> MSAIKPDMKIKLRMEGNVNGHHFVIDGDGTGKPFEGKQSMDLEVKEGGPLPFAFDILTTAFXNRVFAKYPDNIQDYFKQSFPKGYSWERSLTFEDGGICNARNDITMEGDTFYNKVRFYGTNFPANGPVMQKKTLKWEPSTEKMYVRDGVLTGDVETALLLEGNAHYRCDFRTTYKAKEKGVKLPGAHFVDHCIEILSHDKDYNKVKLYEHAVAHSGLPN

The system studied was a reversibly switchable fluorescent protein (rsFP) which is a representative of a class of proteins that undergo a reversible photolysis reaction from a highly fluorescent “on” state to a weakly fluorescence “off” state. The specific rsFP used, rsKiiro, is a mutant of Skylan-NS33 specifically developed for ultrafast time-resolved crystallographic studies due to its ability to form crystals that diffract to high resolution (∼1.1 Å for single-crystal cryo-MX), high photoswitching quantum yield (∼18% Trans-to-Cis in the crystal), and high protein expression yields. Structurally, rsKiiro is similar to green fluorescent protein (GFP) with an 11-stranded β-barrel surrounding an α helix. The chromophore of rsKiiro is formed from the Ala-Tyr-Gly tripeptide at residue numbers 62–64 in the α helix.

In this study, we probed the light-induced reverse reaction, from the Trans to Cis chromophore conformation, initiated with 2 ms 405 nm pulses at a range of optical flash energy densities (0.1–6.7 mJ/mm2) after the initial Cis-to-Trans photoconversion had been driven to completion using ∼13 mW/mm2 of 473 nm CW illumination. A total of 435,200 images were obtained across 6 laser energy densities at 405 nm of 0, 0.1, 0.53, 1.78, 6.74, and 14.43 mJ/mm2. In the preilluminated (unflashed, 0 mJ/mm2) data, signals of the residual Cis population can be seen. This is due to thermally driven ground state isomerization occurring within the 10 ms duration of the X-ray probe due to laser and X-ray induced heating (discussed in detail below). We conclude that the initial population offset seen in the crystallographic data at 0 mJ/mm2 energy density of the 405 nm illumination is due to increased thermal recovery caused by X-ray induced heating. The crystallographic determination of Cis concentration at zero power density of the 405 nm laser is systematically larger than the spectroscopy-based determination. The difference between the crystallographic and spectroscopic quantifications is assigned to the x-induced heating, which drives population across a 91.5 kJ/mol barrier to reform the Cis state. A clear difference in reaction yield can be seen even when comparing the lowest flash energies (0.00 and 0.10 mJ/mm2), where a difference of 3% population transfer is determined from the shift in the minima.>GSGEGPREPGAAGGAAGGSRDALSLEEILRLYNQPINEEQAWAVCYQCCGSLRAAARRRQPRHRVRSAAQIRVWRDGAVTLAPAADDAGEPPPVAGKLGYSQCMETEVIESLG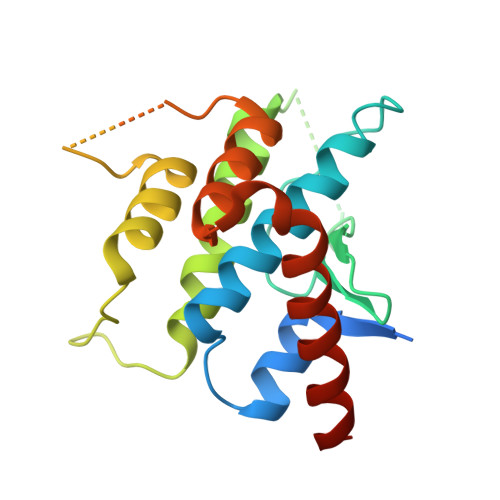IIIYKALDYGLKENEERELSPPLEQLIDHMANTVEADGSNDEGYEAAEEGLGDEDEKRKISAIRSYRDVMKLCAAHLPTESDAPNHYQAVCRALFAETMELHTFLTK[4x]2-(3-phenyloxetan-3-yl)ethanamine | C11 H15 N O | 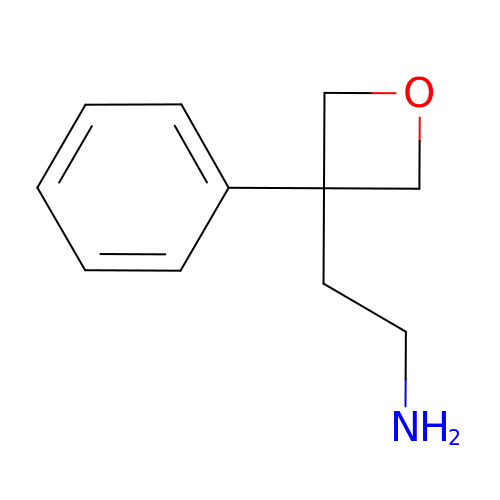WOFYQYBPLNLJAS-UHFFFAOYSA-N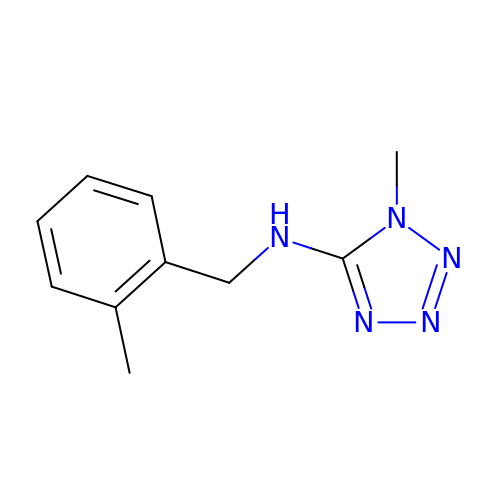1-methyl-N-[(2-methylphenyl)methyl]-1H-tetrazol-5-amine | C10 H13 N5 | CHQPGTNAKZDALZ-UHFFFAOYSA-N> MDISSWFESIHVFLILLNGVFFRL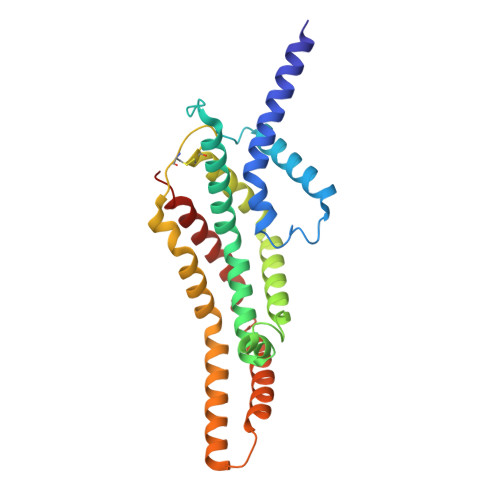APLFFFLPFLNNGIISPSIRIPVIFLVASGLITSGKVDIGSSVFEHVYFLMFKEIIVGLLLSFCLSLPFWIFHAVGSIIDNQRGATLSSSIDPANGVDTSELAKFFNLFSAVVFLYSGGMVFILESIQLSYNICPLFSQCSFRISNILTFLTLLASQAVILASPVMIVLLLSEVLLGVLSRFAPQMNAFSVSLTIKSLLAIFIIFICSSTIYFSKVQFFLGEHKFFTNLFVR>GPGEDDHMEFCRVCKDGGELLCCDACPSSYHLHCLNPPLPEIPNGEWLCPRCTCPPLKGKVQRILHWRWTEPPAPFMVGLPGPDVEPSLPPPKPLEGIPEREFFVKWAGLSYWHCSWVKELQLELYHTVMYRNYQRKNDMDEPPPFDYGSGDEDGKSEKRKNKDPLYAKMEERFYRYGIKPEWMMIH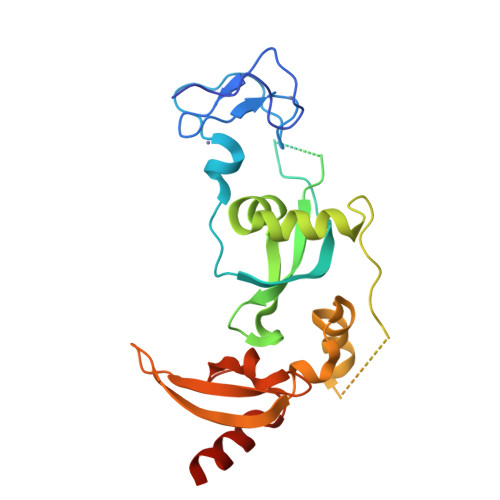RILNHSFDKKGDVHYLIKWKDLPYDQCTWEIDDIDIPYYDNLKQAYWGHRELML[2x]> APSRTLADGDRVPALVIGSGYGGAVAALRLTQAGIPTQIVEMGRSWDTPGSDGKIFCGMLNPDKRSMWLADKTDQPVSNFMGFGINKSIDRYVGVLDSERFSGIKVYQGRGVGGGSLVNGGMAVTPKRNYFEEILPSVDSNEMYNKYFPRANTGLGVNNIDQAWFESTEWYKFARTGRKTAQRSGFTTAFVPNVYDFEYMKKEAAGQVTKSGLGGEVIYGNNAGKKSLDKTYLAQAAATGKLTITTLHRVTKVAPATGSGYSVTMEQIDEQGNVVATKVVTADRVFFAAGSVGTSKLLVSMKAQGHLPNLSSQVGEGWGNNGNIMVGRANHMWDATGSKQATIPTMGIDNWADPTAPIFAEIAPLPAGLETYVSLYLAITKNPERARFQFNSGTGKVDLTWAQSQNQKGIDMAKKVFDKINQKEGTIYRTDLFGVYYK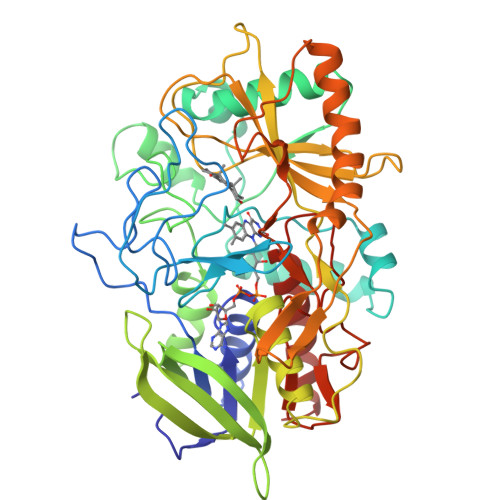TWGDDFTYHPLGGVLLNKATDNFGRLPEYPGLYVVDGSLVPGNVGVNPFVTITALAERNMDKIISSDIQ> GSG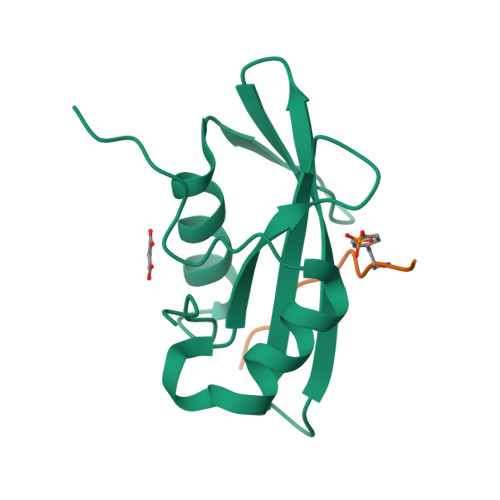RAMDYVDVLNPMPACFYTVSRKEATEMLQKNPSLGNMILRPGSDSRNYSITIRQEIDIPRIKHYKVMSVGQNYTIELEKPVTLPNLFSVIDYFVKETRGNLRPFIASTDENTGQEPSMEGRS;> ANSYENVLIAKX> DRVYIHPFHLVIHNESTCEQLAKANAGKPKDPTFIPAPIQAKTSPVNEKALQDQLVLVAAKLDTEDKLRAAMVGMLANFLGFRIYGMHSELWGVVHGATVLSPTAVFGTLASLYLGALDHTADRLQAILGVPWKDKNCTSRLDAHKVLSALQAVQGLLVAQGRADSQAQLLLSTVVGVFTAPGLHLKQPFVQGLALYTPVVLPRSLDFTELDVAAEKIDRFMQAVTGWKTGCSLMGASVDSTLAFNTYVHFQGKMKGFSLLAEPQEFWVDNSTSVSVPMLSGMGTFQHWSDIQDNFSVTQVPFTESAC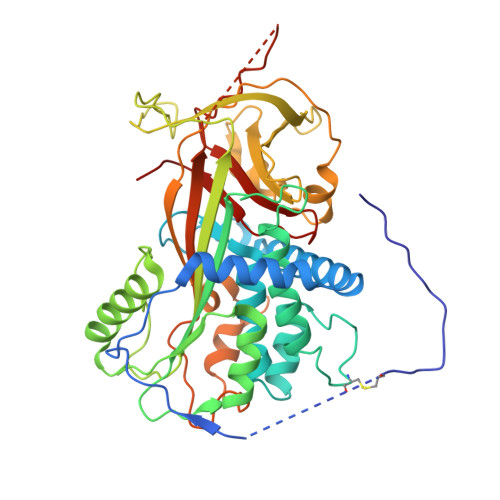LLLIQPHYASDLDKVEGLTFQQNSLNWMKKLSPRTIHLTMPQLVLQGSYDLQDLLAQAELPAILHTELNLQKLSNDRIRVGEVLNSIFFELEADEREPTESTQQLNKPEVLEVTLNRPFLFAVYDQSATALHFLGRVANPLSTA> MSSEPLEPNQDVIIPRSRDSLGRPVYKAQLTRTDNQSEKVALIRQTAPLPVIFIPGIMGTNLRNKADKSEVWRPPNGLWPMDDLFASIGALWTWAWRGPKARQELLKAEQVEVDDQGTIDVGQSGLSEEAARLRGWGKVMRSAYNPVMGLMERRLDNIVSRRELQAWWNDEALSPPGDQGEEQGKVGPIDEEELLRASRYQFDVWCAGYNWLQSNRQSALDVRDYIENTVLPFYQKECGLDPEQMRRMKVILVTHSMGGLVARALTQLHGYERVLGVVHGVQPATGSSTIYHHMRCGYEGIAQVVLGRNAGEVTAIVANSAGALELAPSAEYREGRPWLFLCDAQGQVLKDIDGKPRAYPQNQDPYEEIYKNTTWYGLVPEQNSQYLDMSDKKEGLRVGPRDNFEDLIDSIANFHGELSAAGYHSETYAHYGADDSRHSWRDLIWKGDPTPLETPGATLNDDENGTYNSWFRRGLPTIVQGPLETGNPLDASG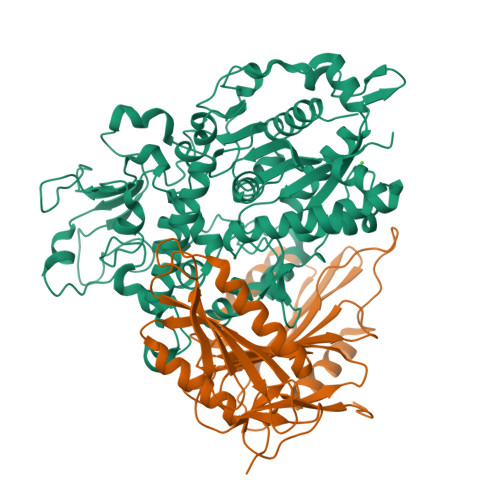SGGDETVPTDSGQAPALAGVKASFRHGSKGKGQANTKRGYEHQESYNDARAQWAALYGVIKITQLADWHPNDKGGT;> MDKTGWITHCFGRFLIDLPPDAVINAGYYLWGDRIEYLDDKPTELAARVDRLEQEWRTQRHKSKGNMFLRKIDFGNESVGLLSWSSEVASKTYLLDTYVTSKPTWHVYRWKGKVSVDREQHAVEISRALARNLRSRAPKEIPSEPGFCIDHAYIAGDSFQVERFGVGVTFPEHPGARFEFRSSTGAELNSLLERVDGFVQNMLSTFAGMETLRKGKHPVGSLPGEEYLVAGSDKGQRGYTFMWEVQGKEESLTEPNLTAGLAVLERSNENGKPPPPAFKSDKEALELWDTIVDSIRVRPTSSSPRGGNAGPSPAPKPATPGGQTLGDHYVYEEFLSSLKPKDSWLDDL>[3x]HGYVESPASRAYQCKLQL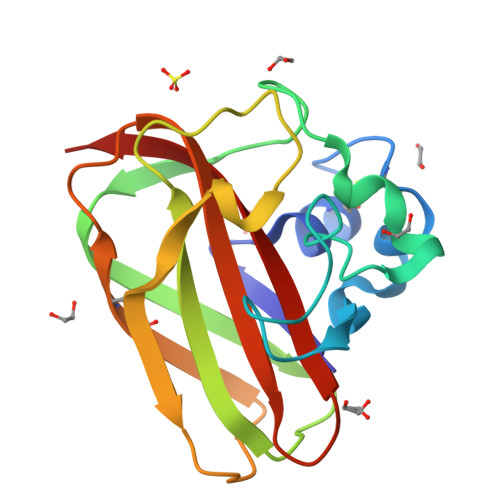NTQCGSVQYEPQSVEGLKGFPQAGPADGHIASADKSTFFELDQQTPTRWNKLNLKTGPNSFTWKLTARHSTTSWRYFITKPNWDASQPLTRASFDLTPFCQFNDGGAIPAAQVTHQCNIPADRSGSHVILAVWDIADTANAFYQAIDVNLSK>MNSLLRLPALKRGVFTMSKRGLATTVSPKTRTSNLKNGLTIASESNPLVQTATVGVWIDAGSRNENAYNNGTAHFFEHLAFKGTDKRSQHQLELDIENMGGHLNAYTSRESTVYYAKSFKDDVPKSVEILADILQHSKLAESAIDREREVITRELEEVNKQYEEVVFDHLHATAFMNQPLGRTILGPRENIQTITNTELRKFITENYTADRMVLVGAGAVDHDALVELAEKYFSHLPSSQSPVPLGTPRSSGEDANQNPIPNFVGSEVRLRDDTMPVAHIAIAVEGVSWTSED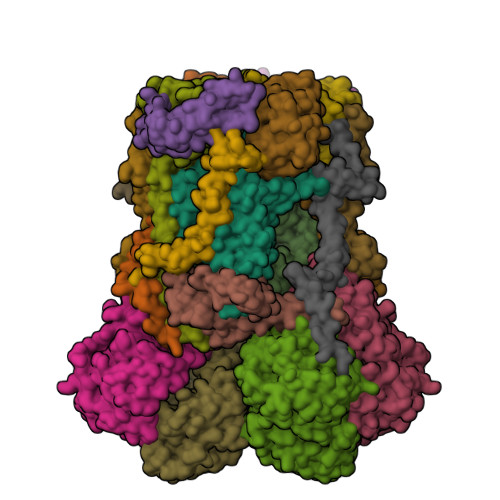YYTALVAQAIIGNYDRAVGTSRHQGSRLSNIVSENNLANSFQSFSTSYSDTGLWGIYLTSENTTQIDDLVHFTLKEWNRLSTSVSNLQVERAKSQLKAGLLLSLDGTTYVAEDIGRQLTTLGRRVTPAEVEAKLEAVTEHDVRAWAQKTLYDKDIALVGLGPIEGLYDYNRIRNDMSMMRW[2x];>MTRGVPRLAVAARHFSTAEAAGVKVAAQDGQSPISDLSVVLRGGSRYATVPGVSHILEKFAFQNTVPKSALRFVRELELFGGKLYTHTTREHIVLRTQFLKQDLPYFVDAFANVLKETKFQQFELTERVAPVAELDLLKRESDPAFTALEAAHEVAFRTGLGNSVYAQGYSPVTLEDVKEFARQVYAKQNVAVVGNNVVPADLQQLVGTAFADLQEGSKVTQAGTTTLHGGEARVRTSTGNALTIALPIAEPKPVYHALASFLGGPASMPWSVGASPLAQATVGTHTSVKATYHNYGDAGLFAITIKGDSPAEISQVAHKAVQALKDTGAEVTEEQAARAYAKSKFAAAEAFENPDSSASVIGMELLSGVSRIAPENVQKFTPAELSEAAAQLSASAKPVVAAVGQVHALPFADELF[2x];>[2x]MALRKKNSLLNMANSYVLDSPQPSNLNYFWNFGSLLALCLVIQLATGITLAMHYTSHASLAFDSVEHIMRDVNFGWFIRYAHANTASFFFICIYAHMGRNIYYGSYKTPRVLPWSIGVIIFLLLIITAFMGYVLVFGQMSLWGATVICNLVSAIPWLGEDIVHFLWGGFSVGNPTLQRFFALHYLMPFVLAVFALLHLIALHTAGSSNPLGITSNVDKLSMHPYYSFKDLITVFAFLLMFTLFVFFSPDKLGHPDNYIPANPMVTPASIVPEWYLLPFYAILRAIPDKLGGVIAMVAAILILLILPIVDRSIIRGNAFKPISKLLFGFFICNFLLLGVLGQVHIEPPFIVLGQICTIFYFSYFLILLPMVSTIENIFFYIGSLRK;>MRRRRIGVWPENRRVSRLWVSLSPRSCVTCPVPTNQNPPINNHHTPILTQMFKAIPLRQALLGISSAVCAGATTTYYYTTKAEAMTAAEHGLHPAEYPWPQNGMLSTFDHASLRRGYQVYKEVCAACHSLDRIAWRNLVGVTHTTDEAKAFAEELEYDDEPDDEGNPRKRPGKLADYIPGPYPNEQAARAANQGALPPDLSLIAKARHGGADYIFALLTGYPDEPPAGVVLAPGMNYNPYFPGGGIGMARTLFDGVVEYEDGTPATTSQMAKDVAAFLTWAAEPEHDERKKLGLKAIIVISAMLGLSVYIKKFKWSPIKNRKFIYNPPKN[2x];>MSLLRTAAQAVKAPKAYTPLVAAKAFAQTRSVSSQPIGGKSTYKIPDFTPYLKKDRNTDANRLFSYFMIGSFGMLSAAGAKATVQDFLSNMSASADVLAMAKVEVKLGAIPLGKNVIIKWRGKPIFIRHRTSEEIEEANEVNVATLRDPQTDDERVQKPEWLVMIGVCTHLGCVPIGEAGDFGGWFCPCHGSHYDISGRIRRGPAPLNLEIPEYDFADAETLVIG[2x];>[2x]MSYFLTLASEVAESLLPTVAFASEEEKEQDEPVEVESDDDESEEKEDDDEEEDEDDDDDDDDDEVPDPAIALHEAAAEGPCHDFKHHFDECVERVTKAQEAEDYDHAEYKEDCVEEFFHLQHCINDNTADKLFRVLK;>[2x]MASITSVVKTSELILKSPLLSKIVVPLAKTYVKFSGYRQLGFKMNDLIIEETPNMQLALRRLPPTESYDRVYRLIRATQFSLSHKLATGNDITKPEEDDHYLIPYILDVEAEAFEKDALDNLEVVKRK;>MGGNGHYMGWWGHMGSPPQKGIAGYTISPFAARPFAGVVHAAIFNTFRRTKNQALFVILPVSFFYYVWTQASEKNEWLYTKAGRHELAKALAE[2x];>[2x]MAWATTFYNVFVKRNSAFVATILASAFVFDMTFETAIDNFWDRINAGKQWKDIRHKYIEAAGDDDEDDE;>[2x]MICGEGDYVKKPSYKIVPHFLGFNIPTVSKWIPIFGIWGAAAGIGALFLIEGVPRTRQDILSKIPIIGEHWIREIPASDNPF>[3x]MKIIKDKVAKLSFVALLVTVTAAMFYTPTASAHGEKSQAAFMRMRTIHWFDLNWSKDQVSVNET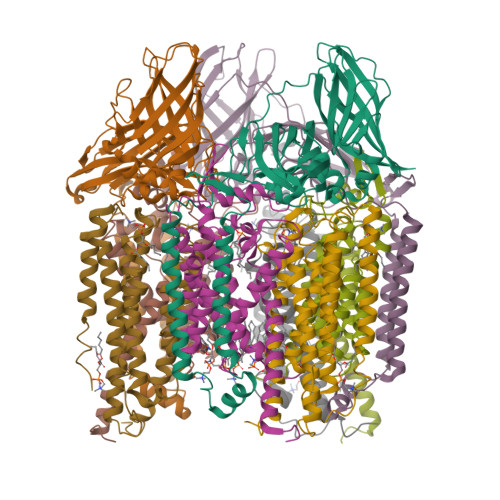MSISGKFHVFAGWPETVDKPEVAFLNIGIPGPVFIRAGSWIGGQLVPRSVSLELGETYEFKVLLKARRPGDWHVHTMMNVQGGGPIIGPGKWVTITGSMGDFKNPITTLTGETIDLETYALDGVYGWHLFWYLLGVAWMVYWCRKPVFIPRRIAVDAGKADSLITPTDKKVGMAFAAGTLAIVAVSMGQANEKYPVTTPLQAGLMRGIKSLELPQPTVSVKVVDASYRVPGRAMQMTLEITNNGDSAVRLAEFNTASVRFLDADVYEDDTNYPDDLLAEEGLSVSDNSPLAPGETRTVDVTASDAAWEVYRLADLIYDPDSRFAGLLFFIDEDGNRQMTMVDAPLIPTFI;>[3x]MSASQSAVRSRAEAVKVSRTFDYMILFTVFFVVLGGYHIHYMLTGGDWDFWTDWKDRRLWVTVAPIVSITFPAAVQAVLWWRYRIAWGATLCVLGLLLGEWINRYFNFWGWTYFPVNFVFPSNLMPGAIVLDVILMLSNSMTLTAVVGGLAWGLLFYPGNWPIIAPLHVPVEYNGMMMTLADLQGYHYVRTGTPEYIRMVEKGTLRTFGKDVAPVSAFFSGFVSILIYFLWHFFGSWFGSEKFVQAA;>MAATTESVKADAAEAPLLNKKNIIAGASLYLVFYAWVRWYEGVYGWSAGLDSFAPEFETYWMNFLYIEMVLEVLVASVLWGYIWKSRDRKVMSITPREELRRHFTHWTWLMMYGIAIYFGASYFTEQDGTWHQTIVRDTDFTPSHIIEFYLSYPIYIITGGASFLYAKTRLPTYQQGLSLQYLVVVVGPFMILPNVGLNEWGHTFWFMEELFVAPLHYGFVFFGWSALGVLGVINIELGALSKLLKKDLA[3x]[2-[(6-oxidanylidene-1~{H}-purin-9-yl)methyl]-3-(phosphonomethoxy)propoxy]methylphosphonic 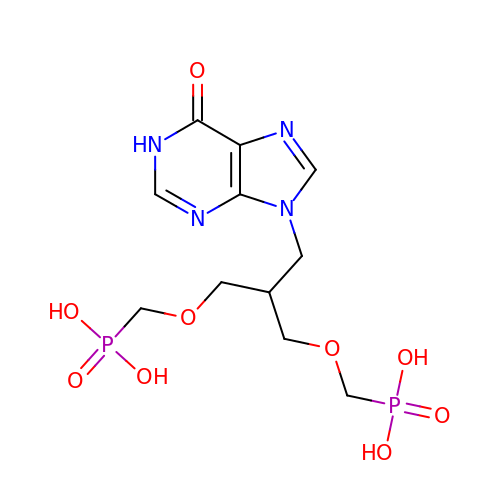acid | C11 H18 N4 O9 P2 | UAIJWVVEDWVBMI-UHFFFAOYSA-N> MPGLSCRFYQHKFPEVEDVVMVNVRSIAEMGAYVSLLEYNNIEGMILLSELSRRRIRSINKLIRIGRNECVVVIRVDKEKGYIDLSKRRVSPEEAIKCEDKFTKSKTVYSIL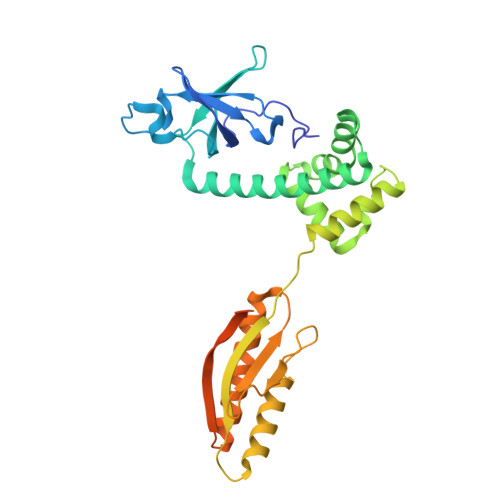RHVAEVLEYTKDEQLESLFQRTAWVFDDKYKRPGYGAYDAFKHAVSDPSILDSLDLNEDEREVLINNINRRLTPQAVKIRADIEVACYGYEGIDAVKEALRAGLNCSTENMPIKINLIAPPRYVMTTTTLERTEGLSVLSQAMAVIKEKIEEKRGVFNVQMEPKVVTDTDETELARQMERLERENAEVDGDDDAEEMEAKAED>[2x]HLNYRQKGVIDVFLHAWKGYRKFAWGHDELKPVSRSFSEWFGLGLTLIDALDTMWILGLRKEFEEARKWVSKKLHFEKDVDVNLFESTIRILGGLLSAYHLSGDSLFLRKAEDFGNRLMPAFRTPSKIPYSDVNIGTGVAHPPRWTSDSTVAEVTSIQLEFRELSRLTGDKKFQEAVEKVTQHI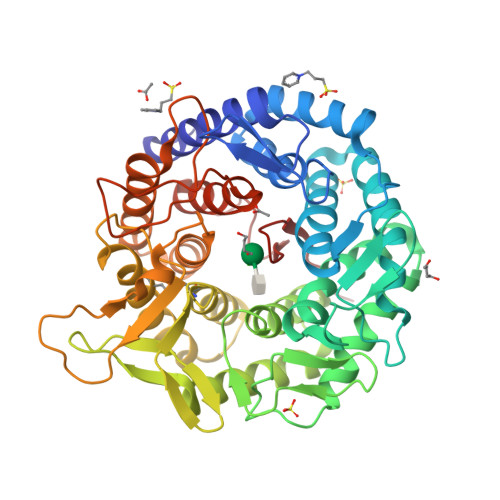HGLSGKKDGLVPMFINTHSGLFTHLGVFTLGARADSYYEYLLKQWIQGGKQETQLLEDYVEAIEGVRTHLLRHSEPSKLTFVGELAHGRFSAKMDHLVCFLPGTLALGVYHGLPASHMELAQELMETCYQMNRQMETGLSPEIVHFNLYPQPGRRDVEVKPADRHNLLRPETVESLFYLYRVTGDRKYQDWGWEILQSFSRFTRVPSGGYSSINNVQDPQKPEPRDKMESFFLGETLKYLFLLFSDDPNLLSLDAYVFNAEAHPLPIWTPA>[4x]AEGGEVDARQRLKEVEVDDNGQFMTTDFGGNIEEQFSLKAGGRGSTLLEDFIFRQKLQHFDHERIPERVVHARGAGAHGIFTSYGDWSNITAASFLGAKDKQTPVFVRFSTVAGSRGSADTARDVHGFATRFYTDEGNFDIVGNNIPVFFIQDAIRFPDLIHSVKPSPDNEVPQAATAHDSAWDFFSSQPSALHTLFWAMSGNGIPRSYRHMDGFGIHTFRLVTEDGKSKLVKWHWKTKQGKAALVWEEAQVLAGKNADFHRQDLWDAIESGNAPSWELAVQLIDEDKAQAYGFDLLDPT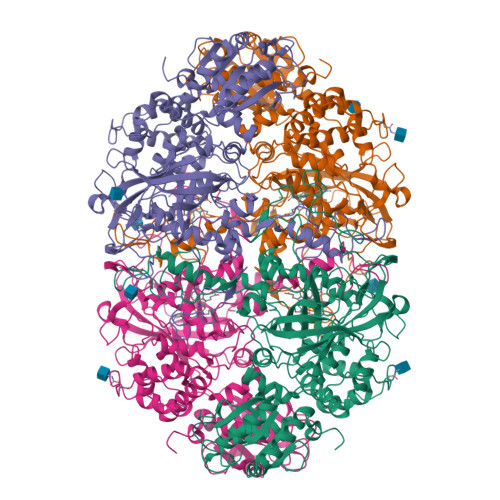KFLPEEFAPLQVLGEMTLNRNPMNYFAETEQISFQPGHIVRGVDFTEDPLLQGRLYSYLDTQLNRHRGPNFEQLPINRPVSGVHNNHRDGQGQAWIHKNIHHYSPSYLNKGYPAQANQTVGRGFFTTPGRTASGVLNRELSATFDDHYTQPRLFFNSLTPVEQQFVINAIRFEASHVTNEQVKKNVLEQLNKISNDVAKRVAVALGLEAPQPDPTYYHNNVTRGVSIFNESLPTIATLRVGVLSTTKGGSLDKAKALKEQLEKDGLKVTVIAEYLASGVDQTYSAADATAFDAVVVAEGAERVFSGKGAMSPLFPAGRPSQILTDGYRWGKPVAAVGSAKKALQSIGVEEKEAGVYAGAQDEVIKGVEEGLKVFKFLERFAVDGDDEE> HMLVLVAPGQGAQTPGFLTDWLALPGAADRVAAWSDAIGLDLAHFGTKADADEIRDTSVAQPLLVAAGILSAAALGTGFTPGAVAGHSVGEI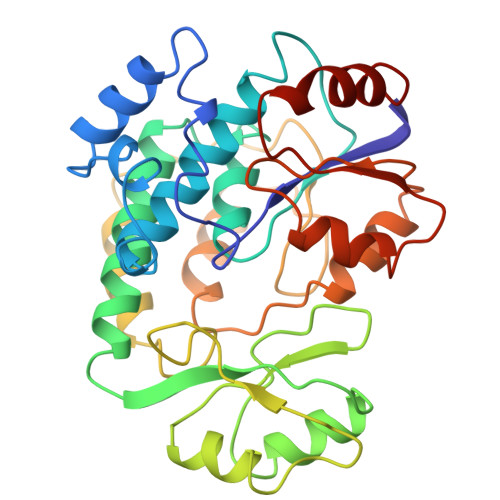TAAVFAGVLDDTAALSLVRRRGLAMAEAAAVTETGMSALLGGDPEVSVAHLERLGLTPANVNGAGQIVAAGTMEQLAALNEDKPEGVRKVVPLKVAGAFHTRHMAPAVDKLAEAAKALTPADPKVTYVSNKDGRAVASGTEVLDRLVGQVANPVRWDLCMETFKELGVTAIIEVCPGGTLTGLAKRALPGVKTLALKTPDDLDAARELVAEHT> ATTLKEAADGAGRDFGFALDPNRLSEAQYKAIADSEFNLVVAENAMKWDATEPSQNSFSFGAGDRVASYAADTGKELYGHTLVWHSQLPDWAKNLNGSAFESAMVNHVTKVADHFEGKVASWDVVNEAFADGGGRRQDSAFQQKLGNGYIETAFRAARAADPTAKLCINDYNVEGINAKSNSLYDLVKDFKARGVPLDCVGFQSH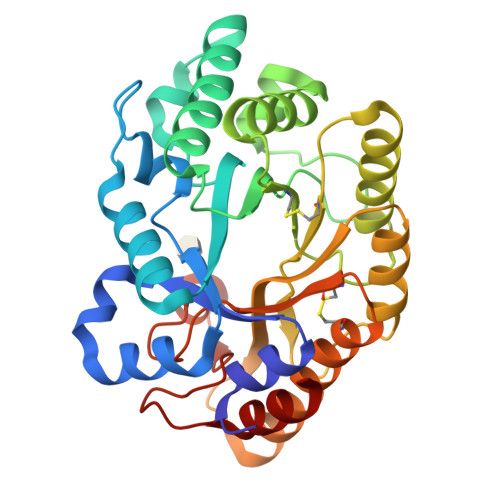LIVGQVPGDFRQNLQRFADLGVDVRITELDIRMRTPSDATKLATQAADYKKVVQACMQVTRCQGVTVWGITDKYSWVPDVFPGEGAALVWDASYAKKPAYAAVMEAF> SNATVDLEQKLEEKFGLEEAIVVATHDMSEEEALNFLAKEAAYTLSKRIAKVKTLGISWGKTIRKFANEFPFIPHKDLTIIPLIGGMG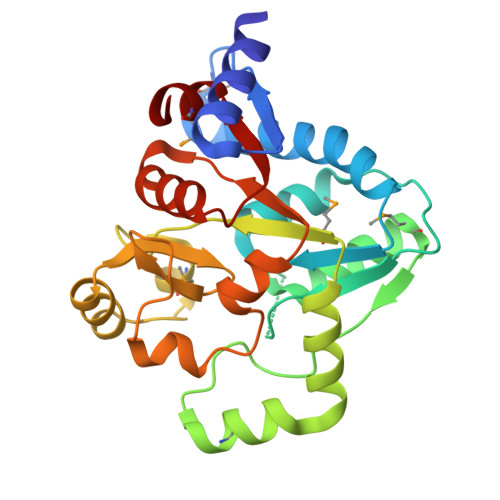SSDIDLHSNQICYDLKKKMKCHSKYLYAPALVEDTEMKTDLSKNKYISEVLEEGKTVDMAIVGVSSPYNHSTMEEIGYINSEDIEELRYKDVVGDINSRFFTADGKEAKTEINTHVIGLSLEELKNIPTVVALANGLQKKEALVAALNAGLIDVIVITDRMAEYIL> GMVEPMTPRFKYTKASQENIQQLGNILEQCFVMSFGDSEIYVKGIGLENFRVIYREQKVAGGLAILPMGQWWGGQRVPMAGIAAVGIAPEYRGDGAAIALIQHTLQEISEQDIPISVLYPATQRLYRKAGYEQAGSSCVWEIP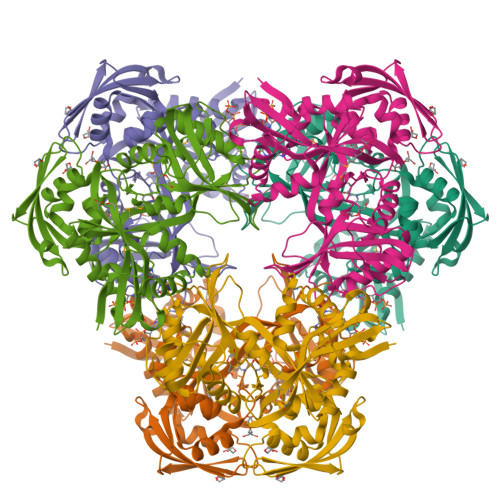TDSIQIQHASLPLEPVVLKNNPIFHELYQQQAQLTHGYLDRHPAIWQGLNRTLDTETLYSYLIGDKDKPQGYIIFTQERTRDGSILRIRDWVTLSNPAVQSFWTFIANHRSQIDKVTWKSSVIDALTLLLPEQSATIRSQDRWMLRIVNVCKALEARGYPLGVEAELHLEVQDDLLATNQGKFILSVANGKSEVTKGGKGELQLDIKGLASLYTSLFTPRQLQLTGKLQATETALLKATQIFAGESPWMIDFF> MSATGPFSIGERVQLTDAKGRRYT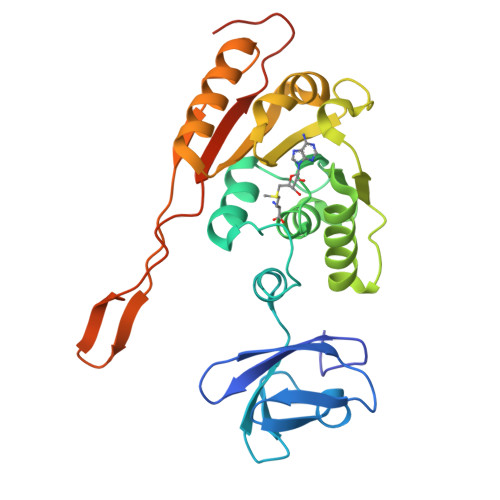MSLTPGAEFHTHRGSIAHDAVIGLEQGSVVKSSNGALFLVLRPLLVDYVMSMPRGPQVIYPKDAAQIVHEGDIFPGARVLEAGAGSGALTLSLLRAVGPAGQVISYEQRADHAEHARRNVSGCYGQPPDNWRLVVSDLADSELPDGSVDRAVLDMLAPWEVLDAVSRLLVAGGVLMVYVATVTQLSRIVEALRAKQCWTEPRAWETLQRGWNVVGLAVRPQHSMRGHTAFLVATRRLAPGAVAPAPLGRKREGRDG>MQLSHHHHHHSSGLVPRGSHMRTQVGIVGAGPAGLMLAHLLRREGIDAVVIERAAREHVRTRLRAGVLEQGTVEMLREAGVGGRIDAVGMEMHAIDFRFGGRSHRLDFHEASGGRRAWVYPQHEVVTDLMSACDAGDVPILYEAPVERIEGLEDDRARIVFGQDGAAGEITCDFVAGCDGFRGVSRGSMPAGIARGYDRIYPFGWLGILADAPPASPDVTWGCSDRGFAMMSMRSPTVTRLYLQCEPDEDPDAWSDDRIWSELHRRLDVEGMPSLREGPIRDKGVTAMRSFLSEPMQHGRLFLAGDAAHIVPPTGAKGLNSAMADIKVLAAALVDHYRHGRSDRLATYSERCLRRMWLVQRFSAALCTMVHQFPGQNEFVRRLQRADLDYMTGTHAGRLQFAENFTGLPIE[4x]

Para-hydroxybenzoate hydroxylase (PHBH) is a group A flavoprotein monooxygenase that hydroxylates p-hydroxybenzoate to protocatechuate (PCA). Among proteins in this clade, Xylophilus ampelinus PobA (XaPobA) preferred PCA as a substrate and is the first known natural PCA 5-hydroxylase (PCAH). The overall structure of XaPobA comprised a homodimer, with each unit binding an oxidized form of FAD in its active site. The XaPobA monomer consisted of FAD-(amino acids 1–73, 88–198, and 267–391)- and substrate (amino acids 74–87 and 199–266)- binding domains.

We initially determined the crystal structure of XaPobA at a resolution of 1.6 Å. An imidazole molecule derived from the crystallization buffer bound to the active site of this structure (XaPobA + imidazole). The imidazole molecule was surrounded by hydrophobic side chains of Val199, Met210, Trp201, and Phe385, and a hydrogen bond was formed with the main chain amide of Thr294. The Arg214 side chain, which anchors the carboxy group of the substrate pHBA in PaPobA, swung out and was not in a conformation suitable for binding to the canonical substrate. The main chain peptide bond of Thr294-Gly295 was notably flipped in the XaPobA + imidazole structure, suggesting that the Thr294‒Gly295 region was flexible due to the absence of hydrogen bond between this region and Cys347, unlike PaPobA.> NNKAGVTYPEIKLGETGKDLKATITFFNGRTDMGLASYPGKNWDAYIKEFNAMYPNITVKVQTDSNYADSALTRLQANNDSWDIMMIPAVDRSEFSNYFVSYGKTEDMDKEIKLANEKAYDGQTYGVATDGQTSGVVYNAKVFKEAGINELPKTPEEFQAALKAIKEKTK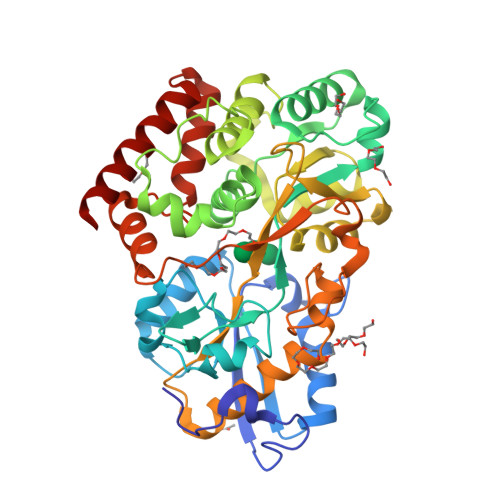AVPLYTNFAEEWAMGAWDQYIGGNATGDPKFMNQIMPHDKTPFAKDDKAPDTHPYAVYKTLYDAVANGYTEEDYSTTDWESSKGKMNNGEIATMVLGAWAVPQMKQAGEHADDVQYMPFPITVDGKQYATLAGNYSMGINKNSDKDRQEAAMIFVKWMTEKSGYSKNEGGIPIVKNDDSYPDTYEHFKDVELIVDAPAKEGEEDLFADINSDSELGINNGNGKKIQDIVVDAANKTKTIDQIMGEWDQKWGKAVESE>MAASGLDHLKNGYRRRFCRPSRARDINTEQGQNVLEILQDCFEEKSLANDFSTNSTKSVPNSTRKIKDTCIQSPSKECQKSHPKSVPVSSKKKEASLQFVVEPSEATNRSVQAHEVHQKILATDVSSKNTPDSKKISSRNINDHHSEADEEFYLSVGSPSVLLDAKTSVSQNVIPSSAQKRETYTFENSVNMLPSSTEVSVKTKKRLNFDDKVMLKKIEIDNKVSDEEDKTSEGQERKPSGSSQNRIRDSEYEIQRQAKKSFSTLFLETVKRKSESSPIVRHAATAPPHSCPPDDTKLIEDEFIIDESDQSFASRSWITIPRKAGSLKQRTISPAESTALLQGRKSREKHHNILPKTLANDKHSHKPHPVETSQPSDKTVLDTSYALIGETVNNYRSTKYEMYSKNAEKPSRSKRTIKQKQRRKFMAKPAEEQLDVGQSKDENIHTSHITQDEFQRNSDRNMEEHEEMGNDCVSKKQMPPVGSKKSSTRKDKEESKKKRFSSESKNKLVPEEVTSTVTKSRRISRRPSDWWVVKSEESPVYSNSSVRNELPMHHNSSRKSTKKTNQSSKNIRKKTIPLKRQKTATKGNQRVQKFLNAEGSGGIVGHDEISRCSLSEPLESDEADLAKKKNLDCSRSTRSSKNEDNIMTAQNVPLKPQTSGYTCNIPTESNLDSGEHKTSVLEESGPSRLNNNYLMSGKNDVDDEEVHGSSDDSKQSKVIPKNRIHHKLVLPSNTPNVRRTKRTRLKPLEYWRGERIDYQGRPSGGFVISGVLSPDTISSKRKAKENIGKVNKKSNKKRICLDNDERKTNLMVNLGIPLGDPLQPTRVKDPETREIILMDLVRPQDTYQFFVKHGELKVYKTLDTPFFSTGKLILGPQEEKGKQHVGQDILVFYVNFGDLLCTLHETPYILSTGDSFYVPSGNYYNIKNLRNEESVLLFTQIKR[2x];> MEEQPQMQDADEPADSGGEGRAGGPPQVAGAQAACSEDRMTLLLRLRAQTKQQLLEYKSMVDASEEKTPEQIMQEKQIEAKIEDLENEIEEVKVAFEIKKLALDRMRLSTALKKNLEKISRQSSVLMDNMKHLLELNKLIMKSQQESWDLEEKLLDIRKKRLQLKQASESKLLEIQTEKNKQKIDLDSMENSERIKIIRQNLQMEIKITTVIQHVFQNLILGSKVNWAEDPALKEIVLQLEKNVDMM;> MSPQKRVKNVQAQNRTSQGSSSFQTTLSAWKVKQDPSNSKNISKHGQNNPVGDYEHADDQAEEDALQMAVGYFEKGPIKASQNKDKTLEKHLKTVENVAWKNGLASEEIDILLNIALSGKFGNAVNTRILKCMIPATVISEDSVVKAVSWLCVGKCSGSTKVLFYRWLVAMFDFIDRKEQINLLYGFFFASLQDDALCPYVCHLLYLLTKKENVKPFRVRKLLDLQAKMGMQPHLQALLSLYKFFAPALISVSLPVRKKIYFKNSENLWKTALLAVKQRNRGPSPEPLKLMLGPANVRPLKRKWNSLSVIPVLNSSSYTKECGKKEMSLSDCLNRSGSFPLEQLQSFPQLLQNIHCLELPSQMGSVLNNSLLLHYINCVRDEPVLLRFYYWLSQTLQEECIWYKVNNYEHGKEFTNFLDTIIRAECFLQEGFYSCEAFLYKSLPLWDGLCCRSQFLQLVSWIPFSSFSEVKPLLFDHLAQLFFTSTIYFKCSVLQSLKELLQNWLLWLSMDIHMKPVTNSPLETTLGGSMNSVSKLIHYVGWLSTTAMRLESNNTFLLHFILDFYEKVCDIYINYNLPLVVLFPPGIFYSALLSLDTSILNQLCFIMHRYRKNLTAAKKNELVQKTKSEFNFSSKTYQEFNHYLTSMVGCLWTSKPFGKGIYIDPEILEKTGVAEYKNSLNVVHHPSFLSYAVSFLLQESPEERTVNVSSIRGKKWSWYLDYLFSQGLQGLKLFIRSSVHHSSIPRAEGINCNNQY;> MNQEDLDPDSTTDVGDVTNTEEELIRECEEMWKDMEECQNKLSLIGTETLTDSNAQLSLLIMQVKCLTAELSQWQKKTPETIPLTEDVLITLGKEEFQKLRQDLEMVLSTKESKNEKLKEDLEREQRWLDEQQQIMESLNVLHSELKNKVETFSESRIFNELKTKMLNIKEYKEKLLSTLGEFLEDHFPLPDRSVKKKKKNIQESSVNLITLHEMLEILINRLFDVPHDPYVKISDSFWPPYVELLLRNGIALRHPEDPTRIRLEAFHQ;> MDSYSAPESTPSASSRPEDYFIGATPLQKRLESVRKQSSFILTPPRRKIPQCSQLQEDVDPQKVAFLLHKQWTLYSLTPLYKFSYSNLKEYSRLLNAFIVAEKQKGLAVEVGEDFDIKVIFSTLLGMKGTQRDPEAFLVQIVSKSQLPSENREGKVLWTGWFCCVFGDSLLETVSEDFTCLPLFLANGAESNTAIIGTWFQKTFDCYFSPLAINAFNLSWMAAMWTACKMDHYVATTEFLWSVPCSPQSLDISFAIHPEDAKALWDSVHKTPGEVTQEEVDLFMDCLYSHFHRHFKIHLSATRLVRVSTSVASAHTDGKIKILCHKYLIGVLAYLTELAIFQIE;> MSVLRPLDKLPGLNTATILLVGTEDALLQQLADSMLKEDCASELKVHLAKSLPLPSSVNRPRIDLIVFVVNLHSKYSLQNTEESLRHVDASFFLGKVCFLATGAGRESHCSIHRHTVVKLAHTYQSPLLYCDLEVEGFRATMAQRLVRVLQICAGHVPGVSALNLLSLLRSSEGPSLEDL;> MDETVAEFIKRTILKIPMNELTTILKAWDFLSENQLQTVNFRQRKESVVQHLIHLCEEKRASISDAALLDIIYMQFHQHQKVWDVFQMSKGPGEDVDLFDMKQFKNSFKKILQRALKNVTVSFRETEENAVWIRIAWGTQYTKPNQYKPTYVVYYSQTPYAFTSSSMLRRNTPLLGQALTIASKHHQIVKMDLRSRYLDSLKAIVFKQYNQTFETHNSTTPLQERSLGLDINMDSRIIHENIVEKERVQRITQETFGDYPQPQLEFAQYKLETKFKSGLNGSILAEREEPLRCLIKFSSPHLLEALKSLAPAGIADAPLSPLLTCIPNKRMNYFKIRDK;> MEQANPLRPDGESKGGVLAHLERLETQVSRSRKQSEELQSVQAQEGALGTKIHKLRRLRDELRAVVRHRRASVKACIANVEPNQTVEINEQEALEEKLENVKAILQAYHFTGLSGKLTSRGVCVCISTAFEGNLLDSYFVDLVIQKPLRIHHHSVPVFIPLEEIAAKYLQTNIQHFLFSLCEYLNAYSGRKYQADRLQSDFAALLTGPLQRNPLCNLLSFTYKLDPGGQSFPFCARLLYKDLTATLPTDVTVTCQGVEVLSTSWEEQRASHETLFCTKPLHQVFASFTRKGEKLDMSLVS;> MDAELAEVRALQAEIAALRRACEDPPAPWEEKSRVQKSFQAIHQFNLEGWKSSKDLKNQLGHLESELSFLSTLTGINIRNHSKQTEDLTSTEMTEKSIRKVLQRHRLSGNCHMVTFQLEFQILEIQNKERLSSAVTDLNIIMEPTECSELSEFVSRAEERKDLFMFFRSLHFFVEWFEYRKRTFKHLKEKYPDAVYLSEGPSSCSMGIRSASRPGFELVIVWRIQIDEDGKVFPKLDLLTKVPQRALELDKNRAIETAPLSFRTLVGLLGIEAALESLIKSLCAEENN;> MSGKANASKKNAQQLKRNPKRKKDNEEVVLSENKVRNTVKKNKNHLKDLSSEGQTKHTNLKHGKTAASKRKTWQPLSKSTRDHLQTMMESVIMTILSNSIKEKEEIQYHLNFLKKRLLQQCETLKVPPKKMEDLTNVSSLLNMERARDKANEEGLALLQEEIDKMVETTELMTGNIQSLKNKIQILASEVEEEEERVKQMHQINSSGVLSLPELSQKTLKAPTLQKEILALIPNQNALLKDLDILHNSSQMKSMSTFIEEAYKKLDAS;> MPVKRSLKLDGLLEENSFDPSKITRKKSVITYSPTTGTCQMSLFASPTSSEEQKHRNGLSNEKRKKLNHPSLTESKESTTKDNDEFMMLLSKVEKLSEEIMEIMQNLSSIQALEGSRELENLIGISCASHFLKREMQKTKELMTKVNKQKLFEKSTGLPHKASRHLDSYEFLKAILN;> MEEEAETEEQQRFSYQQRLKAAVHYTVGCLCEEVALDKEMQFSKQTIAAISELTFRQCENFAKDLEMFARHAKRTTINTEDVKLLARRSNSLLKYITDKSEEIAQINLERKAQKKKKSEDGSKNSRQPAEAGVVESEN;> MADHNPDSDSTPRTLLRRVLDTADPRTPRRPRSARAGARRALLETASPRKLSGQTRTIARGRSHGARSVGRSAHIQASGHLEEQTPRTLLKNILLTAPESSILMPESVVKPVPAPQAVQPSRQESSCGSLELQLPELEPPTTLAPGLLAPGRRKQRLRLSVFQQGVDQGLSLSQEPQGNADASSLTRSLNLTFATPLQPQSVQRPGLARRPPARRAVDVGAFLRDLRDTSLAPPNIVLEDTQPFSQPMVGSPNVYHSLPCTPHTGAEDAEQAAGRKTQSSGPGLQKNSPGKPAQFLAGEAEEVNAFALGFLSTSSGVSGEDEVEPLHDGVEEAEKKMEEEGVSVSEMEATGAQGPSRVEEAEGHTEVTEAEGSQGTAEADGPGASSGDEDASGRAASPESASSTPESLQARRHHQFLEPAPAPGAAVLSSEPAEPLLVRHPPRPRTTGPRPRQDPHKAGLSHYVKLFSFYAKMPMERKALEMVEKCLDKYFQHLCDDLEVFAAHAGRKTVKPEDLELLMRRQGLVTDQVSLHVLVERHLPLEYRQLLIPCAYSGNSVFPAQ;> MAPRGRRRPRPHRSEGARRSKNTLERTHSMKDKAGQKCKPIDVFDFPDNSDVSSIGRLGENEKDEETYETFDPPLHSTAIYADEEEFSKHCGLSLSSTPPGKEAKRSSDTSGNEASEIESVKISAKKPGRKLRPISDDSESIEESDTRRKVKSAEKISTQRHEVIRTTASSELSEKPAESVTSKKTGPLSAQPSVEKENLAIESQSKTQKKGKISHDKRKKSRSKAIGSDTSDIVHIWCPEGMKTSDIKELNIVLPEFEKTHLEHQQRIESKVCKAAIATFYVNVKEQFIKMLKESQMLTNLKRKNAKMISDIEKKRQRMIEVQDELLRLEPQLKQLQTKYDELKERKSSLRNAAYFLSNLKQLYQDYSDVQAQEPNVKETYDSSSLPALLFKARTLLGAESHLRNINHQLEKLLDQG;> MALSTIVSQRKQIKRKAPRGFLKRVFKRKKPQLRLEKSGDLLVHLNCLLFVHRLAEESRTNACASKCRVINKEHVLAAAKVILKKSRG;> MEGAGAGSGFRKELVSRLLHLHFKDDKTKVSGDALQLMVELLKVFVVEAAVRGVRQAQAEDALRVDVDQLEKVLPQLLLDF

The CENP-A nucleosome (CENP-ANuc) is surrounded by a group of 16 proteins, the constitutive centromere-associated network (CCAN) and organized in various stable subcomplexes. Human CCAN is composed by five modules of CENP-C, CENP-LN, CENP-HIKM, CENP-OPQUR and CENP-TWSX. The arrangement of the four sub-complexes generates a b-shaped structure, in which CENP-OPQUR adopts an elongated shape to generate the arm, and CENP-LN, CENP-HIKM, and CENP-TWSX form the semi-circle. The CENP-LN sub-complex, located at the center of the ‘b’, functions as a node for coordination of the assembly of CCAN by contributing the contact sites, with the sub-complexes CENP-HIKM and CENP-OPQU on the opposite side.

We reconstituted a 16-subunit human CCAN complex assembled on CENP-ANuc wrapped with 147 bp of DNA using the Widom 601 sequence. Initial 3D classification and refinement resulted in an EM map with an overall resolution at 3.3 Å of CCAN complex, estimated by the gold-standard Fourier Shell Correlation method. Further classifications and reconstructions gave two maps with distinct features in an interior tunnel, representing the CCAN complex alone (apo-CCAN) and CCAN in complex with a fragment of DNA (CCAN-DNA). The 3.3 Å map was of high quality and was used for model building. The CENP-HIKM sub-complex is comprised of the HIKhead and HIKbase domains connected by the anti-parallel coiled-coil α-helices from CENP-H and CENP-K to form a V-shaped structure. CENP-M, which adopts a small GTPase-like fold, is located at a pocket on the surface of the HIKbase domain formed by the C-terminus of CENP-I, the N-termini of CENP-H and CENP-K, and the CENP-LN sub-complex. At the CENP-QU C-terminal, parallel α-helix bundles, extending in a hetero-dimeric coiled-coil, form the vertical line of “b” with CENP-OP and CENP-R at the top. Although we used a fragment of CENP-C containing amino acid residues 180–545 for reconstitution of CCAN on CENP-A nucleosome, most of this fragment of CENP-C is invisible in the cryo-EM map because of its intrinsic disorder. Assisted by AF2, residues 302–306 of CENP-C were assigned to the density associated with CENP-LN subcomplex in concordance with a previously identified CENP-LN binding motif, which supported the kinetochore recruitment of CENP-LN by CENP-C in vivo. The fragment includes residues 260–272 of CENP-C, which fit into the density proximal to CENP-HIKM subcomplex.>[2x]GSHMTELLKNHVAGQWIAGTGAGITLTDPVTGVALVRVSSEGLDLAR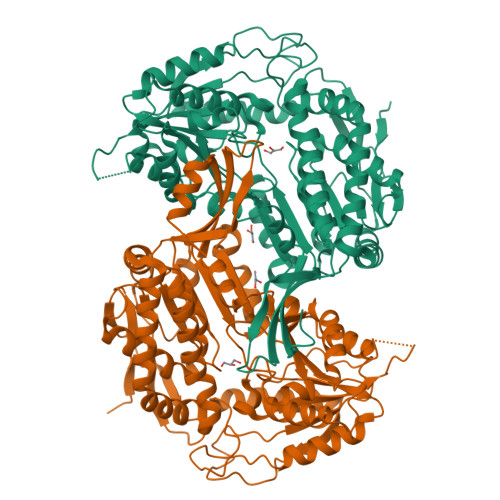AFSFAREDGGAALRALTYAQRAARLADIVKLLQAKRGDYYAIATANSGTTRNDSAVDIDGGIFTLSYYAKLGASLGEVHALRDGSAESLSKDRSFSAQHVLSPTRGVALFINAFNFPSWGLWEKAAPALLSGVPVIVKPATATAWLTQRMVADVVDAGILPPGALSIICGSSAGLLDQIRSFDVVSFTGSADTAATLRAHPAFVQRGARLNVEADSLNSAILCADATPDTPAFDLFIKEVVREMTVKSGQKCTAIRRAFVPEAALEPVLEALKAKLAKITVGNPRNDAVRMGSLVSREQYENVLAGIAALREEAVLAYDSSAVPLIDADANIAACVAPHLFVVNDPDNATLLHDVEVFGPVASVAPYRVTTDTNALPEAHAVALARRGQGSLVASIYSNDDAHLGRLALELADSHGRVHAISPSVQHSQTGHGNVMPMSLHGGPGRAGGGEALGGLRALAFYHRRSAIQAASAAIGTLTQATHWPAA>QQASTLPDLAEQFAPPDVAPPLLIKLVEAIEKKGLECSTLYRTQSSSNPAELRQLLDCDTASLDLEMFDVHVLADAFKRYLLDLPNPVIPVAVSSELISLAPEVQSSEEYIQLLKKLIRSPSIPHQYWLTLQYLLKHFFKLSQTSSKNLLNARVLSELFSPLLFRFPAASSENT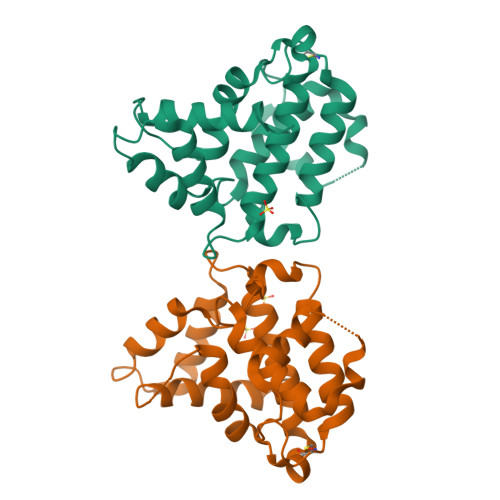EHLIKIIEILISTEWNERQ[2x]>[2x]RDHRKIGKQLDLYHMQEEAPGMVFWHNDGWTIFRE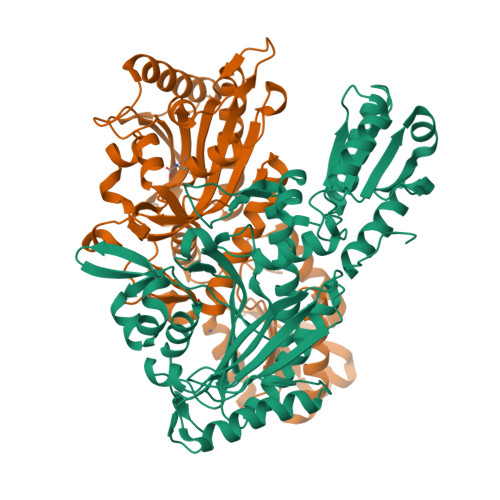LEVFVRSKLKEYQYQEVKGPFMMDRVLWEKTGHWDNYKDAMFTTSSENREYCIKPMNCPGHVQIFNQGLKSYRDLPLRMAEFGSCHRNEPSGSLHGLMRVRGFTQDDAHIFCTEEQIRDEVNGCIRLVYDMYSTFGFEKIVVKLSTRPEKRIGSDEMWDRAEADLAVALEENNIPFEYQLGEGAFYGPKIEFTLYDCLDRAWQCGTVQLDFSLPSRLSASYVGEDNERKVPVMIHRAILGSMERFIGILTEEFAGFFPTWLAPVQVVIMNITDSQSEYVNELTQKLSNAGIRVKADLRNEKIGFKIREHTLRRVPYMLVCGDKEVESGKVAVRTRRGKDLGSMDVNEVIEKLQQEIRSRSLKQLEE>[2x]MDYKDDDDKMHPPETTTKMASVRFMVTPTKIDDIPGLSDTSPDLSSRSSSRVRFSSRESVPETSRSEPMSEMSGATTSLATVALDPPSDRTSHPQDVIEDLSQNSITGEHSQLLDDGHKKARNAYLNNSNYEEGDEYFDKNLALFEEEMDTRPKVSSLLNRMANYTNLTQGAKEHEEAENITEGKKKPTKTPQMGTFMGVYLPCLQNIFGVILFLRLTWVVGTAGVLQAFAIVLICCCCTMLTAISMSAIATNGVVPAGGSYFMISRALGPEFGGAVGLCFYLGTTFAAAMYILGAIEIFLVYIVPRAAIFHSDDALKESAAMLNNMRVYGTAFLVLMVLVVFIGVRYVNKFASLFLACVIVSILAIYAGAIKSSFAPPHFPVCMLGNRTLSSRHIDVCSKTKEINNMTVPSKLWGFFCNSSQFFNATCDEY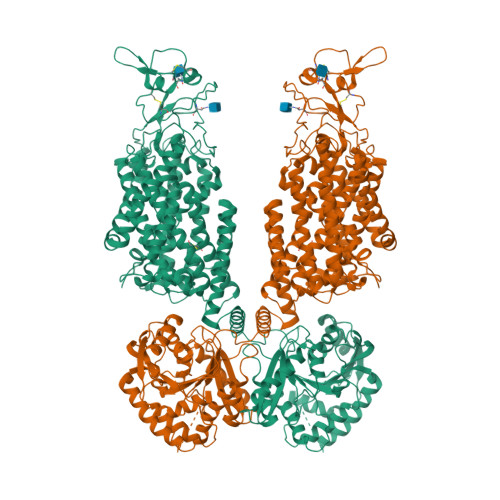FVHNNVTSIQGIPGLASGIITENLWSNYLPKGEIIEKPSAKSSDVLGSLNHEYVLVDITTSFTLLVGIFFPSVTGIMAGSNRSGDLKDAQKSIPIGTILAILTTSFVYLSNVVLFGACIEGVVLRDKFGDAVKGNLVVGTLSWPSPWVIVIGSFFSTCGAGLQSLTGAPRLLQAIAKDNIIPFLRVFGHSKANGEPTWALLLTAAIAELGILIASLDLVAPILSMFFLMCYLFVNLACALQTLLRTPNWRPRFRYYHWALSFMGMSICLALMFISSWYYAIVAMVIAGMIYKYIEYQGAEKEWGDGIRGLSLSAARFALLRLEEGPPHTKNWRPQLLVLLKLDEDLHVKHPRLLTFASQLKAGKGLTIVGSVIVGNFLENYGEALAAEQTIKHLMEAEKVKGFCQLVVAAKLREGISHLIQSCGLGGMKHNTVVMGWPNGWRQSEDARAWKTFIGTVRVTTAAHLALLVAKNISFFPSNVEQFSEGNIDVWWIVHDGGMLMLLPFLLKQHKVWRKCSIRIFTVAQLEDNSIQMKKDLATFLYHLRIEAEVEVVEMHDSDISAYTYERTLMMEQRSQMLRHMRLSKTERDREAQLVKDRNSMLRLTSIGSDEDEETETYQEKVHMTWTKDKYMASRGQKAKSMEGFQDLLNMRPDQSNVRRMHTAVKLNEVIVNKSHEAKLVLLNMPGPPRNPEGDENYMEFLEVLTEGLERVLLVRGGGSEVITIYSWSHPQFEK> GSSGVRLWATRQAMLGQVHEVPEGWLIF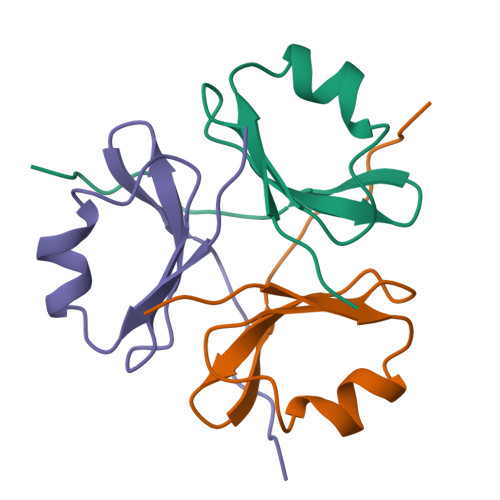VAEQEELYVRVQNGFRKVQLEARTPLPR> IRCFITPDITSKDCPNGHVCYTKTWCDAFCSIRGKRVDLGCAATCPTVKTGVDIQCCSTDNCN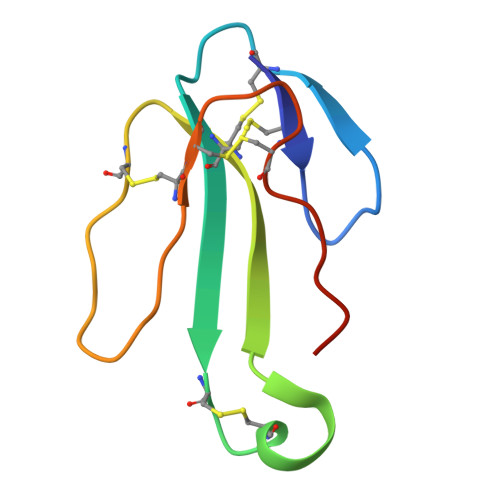PFPTRKRP> GALSPGGTKQKYKEVVDIEAQRRLNDLAREARIRRAQQAVLRKELIATSTNVIKSEISLRILASECHLTLNGIVEAEAQYKMGGLPKSRLPKIKHPMIVTKWVDYSNKHGFSYQLSTEDIGVLFNNGTTVLRLADAEEFWYISYDDREGWVASHYLLSEKPRELSRHLEVVDFFAKYMKANLSRVSTFGREEYHKDDVFLRRYTRYKPFVMFELSDGTFQFNFKDHH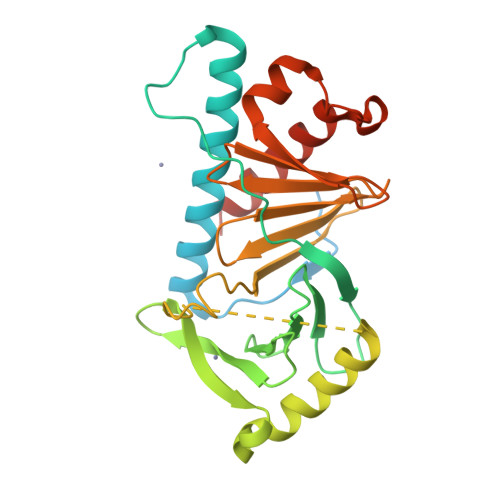KMAISDGGKLVTYISPSHESTTYPLVEVLKYGEIPGYPESNFREKLTLIKEGLKQKSTIVTVD> MESKRNKPGKATGKGKPVGDKWLDDAGKDSGAPIPDRIADKLRDKEFKSFDDFAKAVWEEVSKDPELSKNLNPSNKSSVSKGYSPFTPKNQQVGGRKVYELHHDKPISQGGEVYDMDNIRV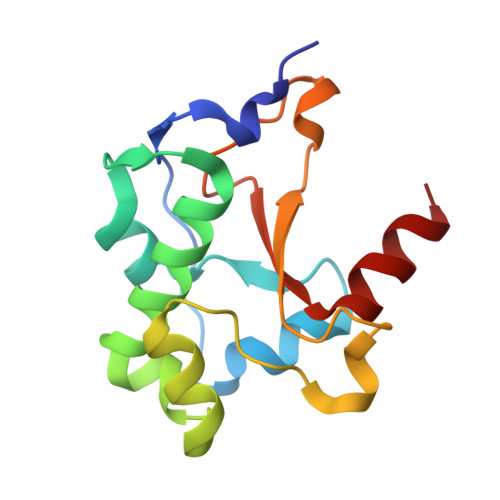TTPKRHIDIHRGK>SMTDEYQLFEELGKGAFSVVRRCMKIPTGQEYAAKIINTKKLSARDHQKLEREARICRLLKHPNIVRLHDSISEEGFHYLVFDLVTGGELFEDIVAREYYSEADASHCIQQILESVNHCHLNGIVHRDLKPENLLLASKSKGAAVKLADFGLAIEVQGDQQAWFGFAGTPGYLSPEVLRKDPYGKPVDMWACGVILYILLVGYPPFWDEDQHRLYQQIKAGAYDFPSPEWDTVTPEAKDLINKMLTINPAKRITASEALKHPWICQRSTVASMMHRQETVDCLKKFNARRKLKGAILTTML[2x]

Calcium/Calmodulin (Ca2+/CaM)-dependent serine/threonine kinases (CaMKs) constitute a family of 81 proteins in the human proteome that play a central role in cellular signaling by transmitting Ca2+ signals. Kinases in this protein family are activated through binding of Ca2+/CaM to regulatory regions that either flank the catalytic domain or are located in regulatory molecules. CaMKII proteins form large oligomeric structures. The N-terminal kinase domain is tethered via an autoinhibitory helix and a calmodulin binding site to a C-terminal oligomerization domain that organizes the enzyme into ring-shaped oligomers.

To address this, we determined the structures of all human CaMKII isozymes in their autoinhibited state. Importantly, whereas the crystallized constructs of the α and β isozymes contained the catalytic domain and the inhibitory region but only a part of the Ca2+/CaM binding motif, the constructs of both CaMKIIγ and CaMKIIδ additionally contained the entire regulatory region as well as a part of the unstructured linker to the association domain. However, the autoinhibitory helices in all isozymes were structured only up to residue 302. Different crystal forms were observed, containing one (CaMKIIγ), two (CaMKIIα and CaMKIIδ), or four molecules (CaMKIIβ) in the asymmetric unit. Similar to the C. elegans orthologue, the substrate binding site is blocked by the regulatory domain in all human CaMKIIs. The sequence flanking T307 represents a site that is incompatible with CaMKII consensus substrate requirements, raising the question as to how this regulatory phosphorylation site would be recognized as a kinase substrate. In the CaMKIIδ structure, T307 was bound to the substrate binding site and oriented in an identical fashion to that observed for T287 in the transphosphorylating complex. The T307-containing region adopts an unusual turn conformation not previously seen in kinase substrate complexes. This unusual binding mode was stabilized by hydrophobic interactions of the conserved residues I304 and L305 that bound inside a deep cavity formed by residues located in the P1 loop and in helix αG.>[4x]MASMSLKHFIQDALSSWMKQKGPESDIVLSSR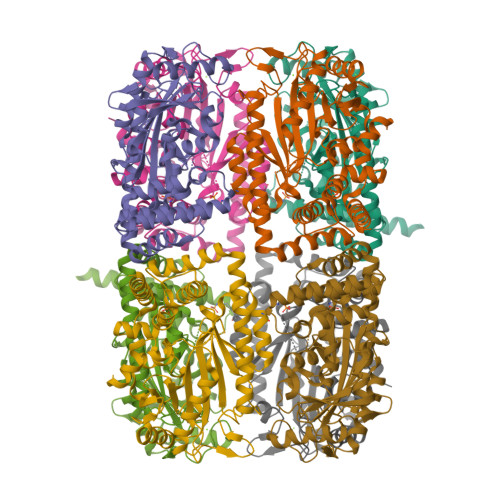IRLARNFEHIRFPTRYSNEEASSIIQQFEDQFSEQEIPGIGKFVLIRMNDAQPLEKRVLVEKHLISPNLTESPFGGCLLSENEEVSVMLNEEDHIRIQCLFPGFQLLEAMKAANQVDDWIEEKVDYAFNEQRGYLTSCPTNVGTGLRASVMMHLPALVLTRQINRIIPAINQLGLVVRGIYGEGSEAVGNIFQISNQITLGKSEQDIVEDLNSVAAQLIEQERSAREAIYQTSKIELEDRVYRSYGVLSNCRMIESKETAKCLSDVRLGIDLGIIKGLSSNILNELMILTQPGFLQQYSGGALRPNERDIRRAALIRERLHLEMNGKRQEDESILEHHHHHH>[6x]MTHHDCAHCSSDACATEMLNLAEANSIETAWH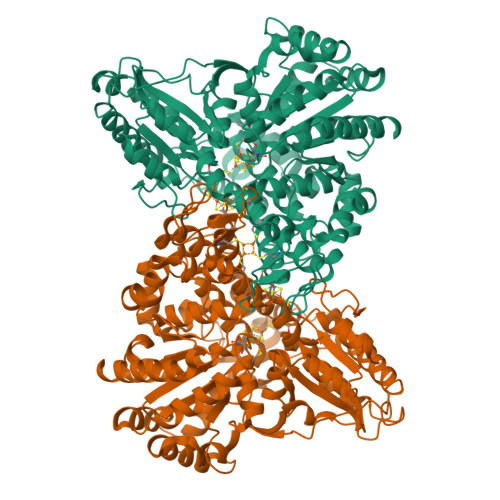RYEKQQPQCGFGSAGLCCRICLKGPCRIDPFGEGPKYGVCGADRDTIVARHLVRMIAAGTAAHSEHGRHIALAMQHISQGELHDYSIRDEAKLYAIAKTLGVATEGRGLLAIVGDLAAITLGDFQNQDYDKPCAWLAASLTPRRVKRLGDLGLLPHNIDASVAQTMSRTHVGCDADPTNLILGGLRVAMADLDGSMLATELSDALFGTPQPVVSAANLGVMKRGAVNIAVNGHNPMLSDIICDVAADLRDEAIAAGAAEGINIIGICCTGHEVMMRHGVPLATNYLSQELPILTGALEAMVVDVQCIMPSLPRIAECFHTQIITTDKHNKISGATHVPFDEHKAVETAKTIIRMAIAAFGRRDPNRVAIPAFKQKSIVGFSAEAVVAALAKVNADDPLKPLVDNVVNGNIQGIVLFVGCNTTKVQQDSAYVDLAKSLAKRNVLVLATGCAAGAFAKAGLMTSEATTQYAGEGLKGVLSAIGTAAGLGGPLPLVMHMGSCVDNSRAVALATALANKLGVDLSDLPLVASAPECMSEKALAIGSWAVTIGLPTHVGSVPPVIGSQIVTKLVTETAKDLVGGYFIVDTDPKSAGDKLYAAIQERRAGLGL>MTRLPKLAVFDLDYTLWPFWVDTHVDPPFHKSSDGTVRDRRGQNIQLYPEVPEVLGRLQSLGVPVAAASRTSEIQGANQLLELFDLGKYFIQREIYPGSKVTHFERLHHKTGVPFSQMVFFDDENRNIIDVGRLGV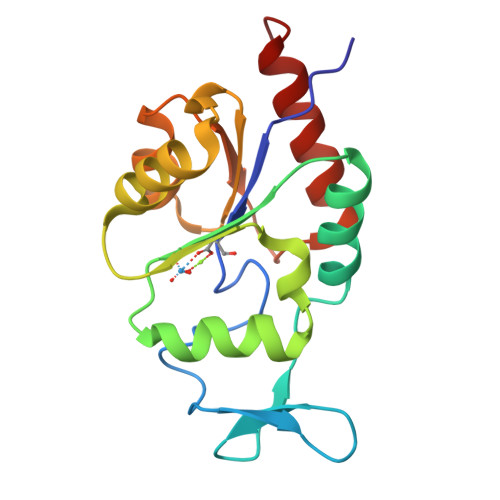TCIHIRDGMSLQTLTQGLETFAKAQAGL[4x]> GQKHEFANYKRYATENAALAQPVKKEKRVVFMGNSI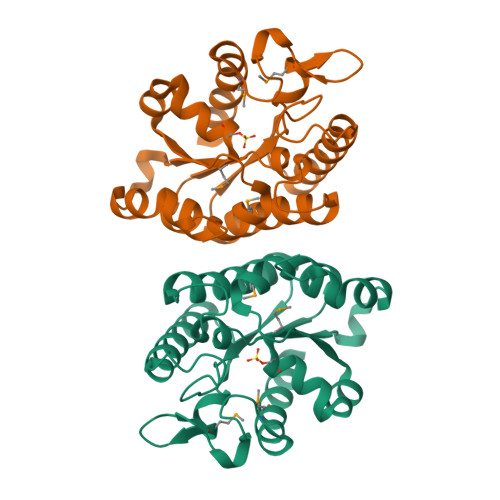TEGWVRTHPDFFKTNGYIGRGISGQTSYQFLLRFREDVINLSPALVVINAGTNDVAENTGAYNEDYTFGNIASMAELAKANKIKVILTSVLPAAEFPWRREIKDAPQKIQSLNARIEAYAKANKIPFVNYYQPMVVGENKALNPQYTKDGVHPTGEGYDIMEALIKQAIEKAL N-(2-isopropoxy-4-(4-methylpiperazine-1-carbonyl)phenyl)-2-(3-(phenylcarbamoyl)phenyl)thiazole-4-carboxamide 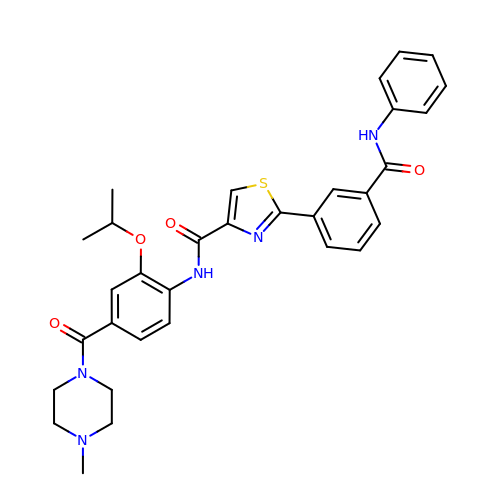| C32 H33 N5 O4 S | CKGXWWJPWNFXBV-UHFFFAOYSA-N> PL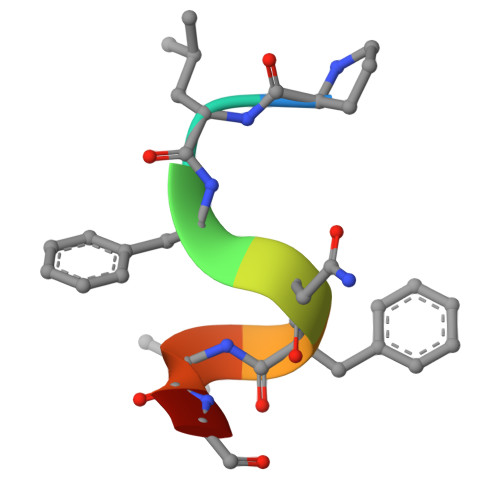FNFLCG>MAHHHHHHHRSAAGTIWEFDGGACGARTALVKVDRVDRRYQDLVTRGFNGRFRGRPDVVYVVHTADQVVDAVNQAMAAGQRIAVRSGGHCFEGFVDDPAVRAVIDMSQMRQVFYDSGKRAFAVEPGATLGETYRALYLDWGVTIPAGVCPQVGVGGHVLGGGYGPLSRRDGVVADHLYAVEVVVV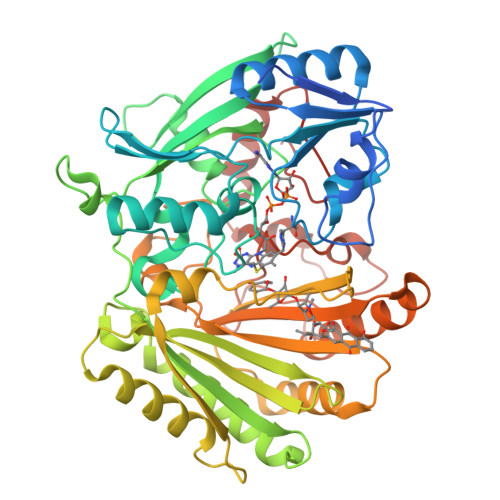DASGRARKVVATSAADDPNRELWWAHTGGGGGNFGIVTRYWFRTPGATGTDPSQLLPKAPTSTLRHIVTWDWSALTEEAFTRIIDNHGAWHQSNSAAGTPYASMHSVFYLNSRAAGQILLDIQIDGGLDGAEALLNDFVAAVNEGTGVEPAVQRSTEPWLRATLANKFDTGGFDRTKSKGAYLRKPWTAAQAATLYRHLSADSQVWGEVSLYSYGGKVNSVPETATATAQRDSIIKVWMSATWMDPAHDDANLAWIREIYREIFATTGGVPVPDDRTEGTFINYPDVDLVDERWNTSGVPWYTLYYKGNYPRLQKVKARWDPRDVFRHALSVRPPG[4x]>MELEIRPLFLVPDTNGFIDHLASLARLLESRKYILVVPLIVINELDGLAKGQETDHRAGGYARVVQEKARKSIEFLEQRFES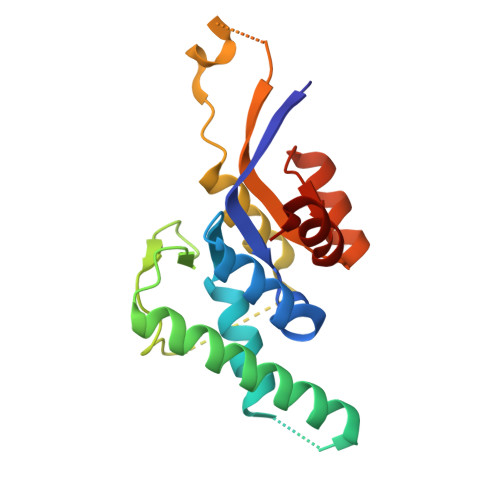RDSCLRALTSRGNELESIAFRSEDITGQLGNNDDLILSCCLHYCKDKAKDFMPASKEEPIRLLREVVLLTDDRNLRVKALTRNVPVRDIPAFLTWAQVG[3x]> MPVITVNTNVAEKSIPVFFQAALTNMMTKALQKPKEVMFVDLRSGANIMMGGDRNPCVFATVECIGRLNP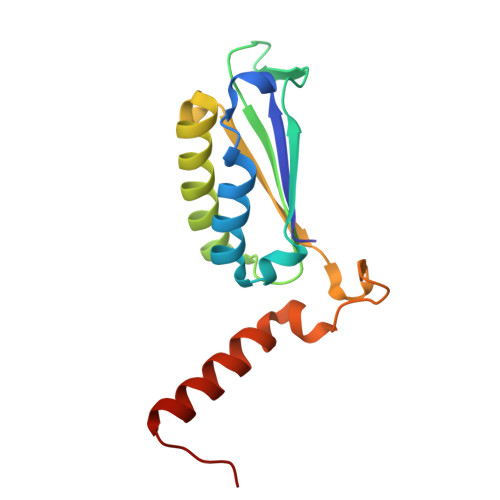TSNLAMARDMEDMFIEHLNVRRERIVIRFIPVPALFCSFNGALHDVSIERDEDIISQAIAEYLHHHHHHHA> MEHNLSPLQQEVLDKYKQLSLDLKALDETIKELNYSQHRQQHSQQETVSPDEILQEMRDIEVKIGL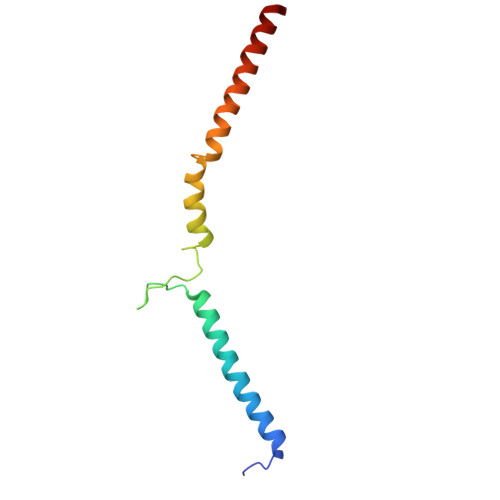VGTLLKGSVYSLILQRKQEQESLGSNSK The BT1062 gene of B. thetaiotaomicron encodes a predicted lipoprotein with a molecular weight of 36 535 Da (residues 1–317) and a calculated isoelectric point of 4.8. BT1062 is a member of a functionally uncharacterized protein family [Pfam PF08842 or DUF1812 (domain of unknown function family 1812)] consisting of ∼80 Bacteroidetes proteins of around 300–400 residues. Therefore, the BT1062–BT1068 genes are most likely to encode a fimbriae (or pili) system similar to that of the minor fimbriae of P. gingivalis, with BT1062 being equivalent to mfa2. Thus, DUF1812 is a collection of diverse proteins that are likely to be fimbrial components.

The selenomethionine derivative of BT1062 (residues 23–317) with an N-terminal His tag was expressed in E. coli and purified by metal-affinity chromatography. The crystal structure of BT1062 was determined in the tetragonal space group P41212 at 2.2 Å resolution using the MAD method. The structure of BT1062 consists of a tandem repeat of two domains: I (34–170) and II (171–317). BT1062 is composed of 21 β-strands (β1–β21), three α-helices (α1–α3) and five 310-helices. BT1062 is likely to exist as a monomer in solution, which is consistent with crystal-packing analysis and analytical size-exclusion chromatography. The most significant additional structural feature of BT1062 is a small β-sheet at the domain boundary formed by the EF loop of domain I and the BC loop of domain II. Domain II contains a three-helix insertion between strands F and G as well as a β-hairpin attachment (β20–β21) at the C-terminus. Most sequence homologs of BT1062 and Mfa2 contain two highly conserved cysteines at the N-terminus (Cys25 and Cys35) located near the tip of the bilobal molecule. The conformation of the peptide between the two conserved cysteines is likely to be flexible since residues 24–33 are exposed to solvent and disordered in the crystal with no interpretable electron density. The most conserved surface residues of BT1062 homologs correspond to a short sequence motif 306N(G/D)W308 located in the β20–β21 loop.

> GASCDSFNEDLPECRLSVKFKYDYNMEFADAFHAQVDKVELYVFDKNGKYLFKQAEEGSALSTGNYLMEVELPVGQYQFMAWAGARDSYDITSLTPGVSTLTDLKLKLKREASLIINKRMETLWYGEVINVNFDGTVHQTETINLIRDTKIVRFGFQSYTGSWTLDMNDYDYEIIESNGHLGHDNSLLDDDVLSFRPYYMEQKDPATAYVDMNTMRLMEDRKTRLVLTEKASGKRVFDINLIDYLAMTNAEGKNLSTQEYLDRQSNYHIIFFLSESWLAVQIVVNGWVHRIQEENQ> KEPEKPIDREKTCPLLLRVFTTNNGRHHRMDEFSRGNVPSSE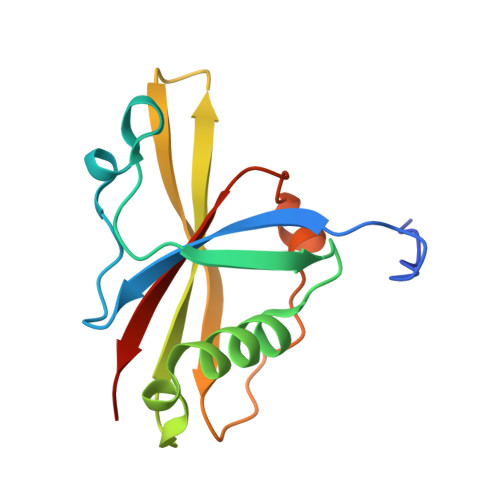LQIYTWMDATLKELTSLVKEVYPEARKKGTHFNFAIVFMDLKRPGYRVKEIGSTMSGRKGTDDSMTLQSQKFQIGDYLDIAITPPNRA>[3x]APAAVDWRARGAVTAVKDQGQCGSSWAFSAIGNVECQWFLAGHPLTNLSEQMLVSCDK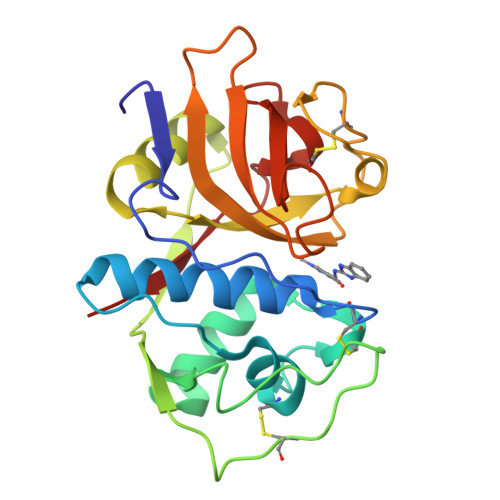TDSGCSGGLMNNAFEWIVQENNGAVYTEDSYPYASGEGISPPCTTSGHTVGATITGHVELPQDEAQIAAWLAVNGPVAVAVDASSWMTYTGGVMTSCVSEQLDHGVLLVGYNDSAAVPYWIIKNSWTTQWGEEGYIRIAKGSNQCLVKEEASSAVVG> MSLSRTQIVNWLTRCGDIFSTESE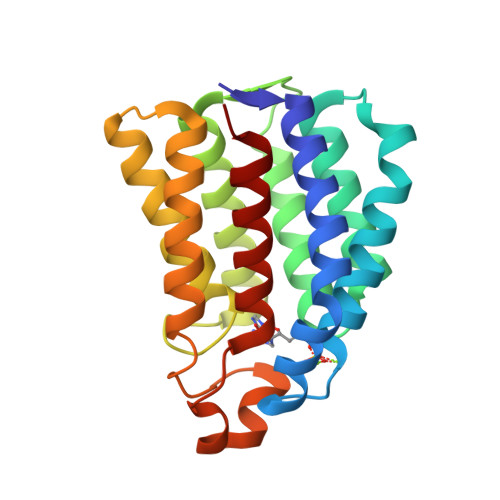YLTGLDREIGDADHGLNMNRGFSKVVEKLPAIADKDIGFILKNTGMTLLSSVGGASGPLFGTFFIRAAQATQARQSLTLEELYQMFRDGADGVISRGKAEPGDKTMCDVWVPVVESLRQSSEQNLSVPVALEAASSIAESAAQSTITMQARKGRASYLGERSIGHQDPGATSVMFMMQMLALAAKE Type VII secretion systems (T7SSs), also referred to as ESAT-6 secretion (ESX) systems, are AAA+-dependent molecular machines that are found in the Actinomycetota phylum and have gained great attention due to their implications in cell homeo­stasis and host–pathogen interactions in mycobacteria. Among them, ESX-5 is found almost exclusively in slow-growing pathogenic mycobacteria, where it participates in nutrient uptake, intracellular colonization and modulation of the immune response during infection through the secretion of a large family of protein effectors: the PE and PPE proteins. EccC is a pivotal component of the pore complex, providing the secretion driving force via the hydrolysis of ATP. In the ESX-2 to ESX-5 systems, EccC consists of two N-terminal transmembrane (TM) helices connected to two additional helices (the stalk region) and a domain of unknown function (EccCDUF), which are followed by three FtsK/SpoIIIE AAA+ ATPase domains, here referred to as D1, D2 and D3 (EccCD1–D3; Famelis et al., 2023; Bunduc et al., 2021).

Here, the crystal structure of the MtbEccC5 DUF domain is reported at 2.05 Å resolution, which reveals a nucleotide-free structure with degenerated cis-acting and trans-acting elements involved in ATP binding and hydrolysis. The core structure consists of a six-stranded parallel β-sheet (β5–β1–β4–β3–β2–β2′) further extended by an additional two-stranded antiparallel sheet (β6–β7). The C-terminal α-helical lid present in other prokaryotic AAA+ domains is missing in the structure, which is flanked by two parallel helices (αA and αB) and a two-stranded antiparallel sheet (βA–βB) that connects to the stalk domain. This structure is conserved in both molecules present in the asymmetric unit (r.m.s.d. of 0.173 Å for 218 Cα atoms). The proposed ATP-binding site should be located at the N-terminus of the α1 helix and the C-terminus of the β3 strand, which are expected to contain the P-loop and the Walker B motif, respectively. Sequence analysis of the Walker A motif shows a highly degenerated and one amino acid shorter sequence (GEREQVL231) that is missing the conserved G2 and G3 glycines as well as the Lys and Thr/Ser residues that are key for ATP/Mg2+ stabilization (Val30 and Leu231 in). Inspection of the crystal model shows an ATP-free structure in which the degenerated Walker A motif folds as an extended α1 helix instead of the standard P-loop conformation. Altogether, this points to variations of G2 and G3 as structural factors responsible for the extended α1 helix observed in . Inspection of the Walker B motif also shows conformational deviations in , which include a shorter β3–α3 loop and a hydrophobic residue (Val329) replacing the catalytic base.

>GPMKRGFARPTPEKPPVIGSSGQESADSMDANYRWFHPAPNTLAAAVGSPRMWERKPDGKDLNFGVVRVGGSGFGRYQSVVYNLPKMVSLLVEPWYALVGEREQVLGLMRAIICQLAFSHGPDHVQMIVVSSDLDQWDWVKWLPHFGDSRRHDAAGNARMVYTSVREFAAEQAELFAGRGSFTPRHASSSAQTPTPHTVIIADVDDPQWEYVISAEGVDGVTFFDLTGSSMWTDIPERKLQFDKTGVIEALPRDRDTWMVIDDKAWFFALTDQVSIAEAEEFAQKLAQWRLA[2x]MmtN is an S-adenosyl-methionine (SAM)-dependent methyltransferase family enzyme. MmtN catalyzes the S-methylation of Met, in which the methyl group of SAM is transferred to the Met molecule to generate SMM. Recently, diverse marine Actinobacteria, α- and γ-proteobacteria were shown to initiate DMSP synthesis via the methionine (Met) S-methyltransferase enzyme (MmtN), generating S-methyl-Met (SMM). We propose that MmtN uses the proximity and desolvation mechanism for Met S-methylation with two adjacent MmtN monomers comprising the Met binding site.

The electron density map of the MmtN-SAM binary complex structure showed that one SAM molecule was positioned in the active-site of each MmtN monomer, mainly through hydrogen bonding interactions. We predict Ser101 and Leu102 form hydrogen bonds with the adenine ring of SAM, whilst SAM also forms hydrogen bonds through both ribose hydroxyls to the side chain carboxyl oxygen of Asp69. The amino group of SAM contacts with the carboxyl group of Glu127 by forming another hydrogen bond. The electron density map of MmtN-SAM binary complex showed that two glycerol molecules were located alongside the reactive methyl group of the SAM molecule, indicating that these two glycerol molecules occupied the Met-binding site. By comparing the structures of the three monomers in the MmtN-SAM binary complex, we found that the conformations of three SAM molecules were slightly different from one another, suggesting that the binding of SAM by MmtN may not be tight. These structural observations are consistent with the biochemical data showing that MmtN had a relatively low affinity for SAM. Moreover, the Helixα5 (Val131-Gln140) shifts ~10o in different monomers. When superimposing the structures of MmtN and the MmtN-SAM complex, we found that Tyr160 formed a loop region (His158-Tyr162) occupying the binding site of the adenine ring of SAM, and the mutation of Tyr160 to alanine greatly increased the Kd of MmtN towards SAM. This loop swings away from the SAM-binding pocket in the MmtN-SAM complex, indicating that it has a gating function for SAM entry. The overall structures of MmtN-SAM and MmtN-SAH-Met were similar to that of MmtN, with a root mean square deviation (RMSD) of 0.27 Å between MmtN and MmtN-SAM complex and of 0.23 Å between MmtN and MmtN-SAH-Met complex.

>[3x]MGDSEEPVVTPHAPEFAFDPTDPWTETFQRGLEIAGLGGKRVYEVGIGTGINVAFMLQICEAALVSGSDLDPRLAGLAERNVRDLAPRRADRFHPVEGAVSLIDTPEARAQVGRSDVIVGCLPQVGEPDDVRLRAFRTAQAAALAAGADTRDEDHIAHYYPWAEFDSYPFNSVGLGLNEALLRRTRATAPAADVVLNFGARVGSAVLFELFEANGYVPEKLHSQIVLQHAGTDISFFVALENALAQTGLEREFTCEFYGDPEGATRLSATEAQALVDTDSAAEIYHEVCVIRGRPALSENDPSDS> GPLGSMSQSNRELVVDFLSYKLSQKGYSWSQMAAVKQALREAGDEFELRYRRAFSDLTSQLHITPGTAYQSFEQVVNELFRDGVNWGRIVAFFSFGGALCVESVDKEMQVLVSRIAAWMATYLNDHLEPWIQENGGWDTFVELYGNNAAAESRKGQER;> XWIAQELREIGDKFN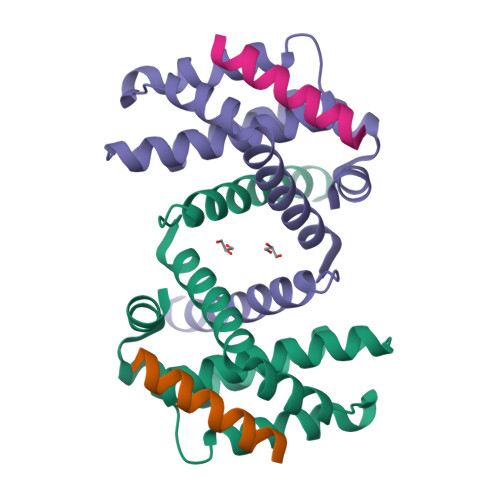AYYAX> MAPVKVFGPAMSTNVARVTLCLEEVGAEYEVVNIDFNTMEHKSPEHLARNPFGQIPAFQDGDLLLWESRAISKYVLRKYKTDEVDLLRESNLEEAAMVDVWTEVDAHTYNPALSPIVSQCLFNPMMRGLPTDEKVVAESLEKLKKVLEVYEARLSKHSYLAGDFVSFADLNHFPYTFYFMATPHAALFDSYPHVKAWWDRLMARPAVKKIAATMVPPKA

In black-grass, upregulation of a phi (F)-class GST1 (AmGSTF1) has been shown to be a functional biomarker of MHR. Recombinant AmGSTF1 has been shown to exhibit both glutathione-S-transferase activity toward xenobiotics, as well as acting as a GPOX, reducing fatty-acid hydroperoxides to less reactive monohydroxy derivatives. The Phi (F) class GSTs, of which AmGSTF1 is an example, are found in all higher plants, being homodimeric enzymes in which each protomer of approximately 23–30 kDa with the catalytic serine residues located at the interface. Each protomer has two distinct domains; the N-terminal domain adopts the typical thioredoxin-fold, with the C-terminal domain being a bundle of at least five helices as demonstrated by the crystal structures of AmGSTF1 presented here.

In spite of extensive crystallisation and soaking efforts, no crystal with any substrate bound or any alternative crystal packing forms of the wild-type protein were obtained. Based on a careful analysis of the crystal packing, the key hydrophobic contact stabilising a crystallographic dimer interface shown in Fig. 1b was identified and three protein variants were designed to facilitate alternative packing. The Phe122Tyr variant therefore adopted the closed conformation for the two loops over the binding cleft with glutathione bound in the G-site. Having identified new crystallisation conditions for the Phe122Thr variant, a similar approach was used in screening for the Tyr118Ser AmGSTF1 variant, with the structure determined to a resolution of 2.6 Å (Table S1b‡). Density was observed again associated with a glutathione molecule in the binding site, although this was refined with a reduced occupancy of 0.7. Interestingly, the Tyr118Ser mutation resulted in the top of the α4 helix becoming disordered, with the weak density observed for residues from Phe122 to Thr131 consistent with considerable flexibility. This suggests that interactions formed by this Tyr118 residue are essential to the structure of this helix and may explain the reduced enzymatic activity associated with the mutation of this residue.> MAVPFVEDWDLVQTLGEGSFGEVQLAVNRVTEEAVAVKIVDMKRAVDCPENIKKEICILKMLNHENVIKFYGHRREGNIQYLFMELASGGSLFDRIEPDIGMPEPDAQRFFHQLMAGVVYLHGIGITHRDIKPHNLLLDERDNLKIADYSLATVFRYNNRERLLNKMCGTLPYVAPELLKRREFHAEPVDVWSCGIVLTAMLAGELPWDQPSDSCQEYSDWKEKKTYLNPWKKIDSAPLALLHKILVENPSARITIPDIKKDRWYNKPLKKGAKRPRVTSGGV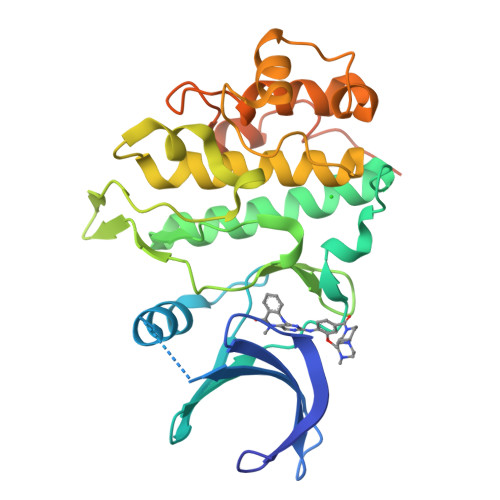SESPSGHHHHHHHH>SEFMLDFDLVLFGATGDLAMRKLFVSLYEIYTHYGFKKDSKIIASGRKELSNEEFLALLCEKTQLHSREKGEEFLAHISYFCVRLDNPKDFEELSKIATKNKPLIFYFSISPSFFTTTAQNLAQNALNHANTRLILEKPLGHDLKTCKEIFQSISAFFKEEQIFRIDHYLGKKGVQNILELRLNNPILNILWDQISAVEICVYETLGVEERGEFYDKIGALRDMVQNHLLQVLSLIATDLPDDLKDLRKEKIKVLKTLQPPKNF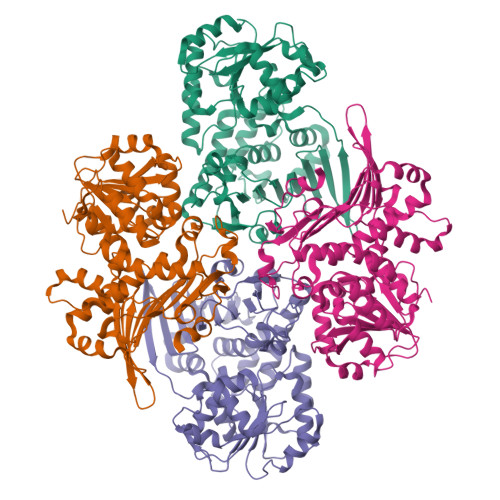KKQVIRAQYQGYRDENKVNKESQTETFVAIKAFLDTPKFKGVPFYLKHAKKMPHNQASVKIHFNAVNTLEFFLSQDKITLTLKDHQNPLILETYNKQEFLQPYAKLLYDAIQNNHNNFAHQLELEASWVFIDTLIEGFINNATPLYSYESHNLNESEFLKPLYQ[4x]>MNVDPHFDKFMESGIRHVYMLFENKSVESSEQFYSFMRTTYKNDPCSSDFECIERGAEMAQSYARIMNIKLETE[4x];>[4x]MEYYKQSKYETYSEIIEKERTARFESVALEQLQIVHISSEADFSAVYSFRPKNLNYFVDIIAYEGKLPSTISEKSLGGYPVDKTMDEYTV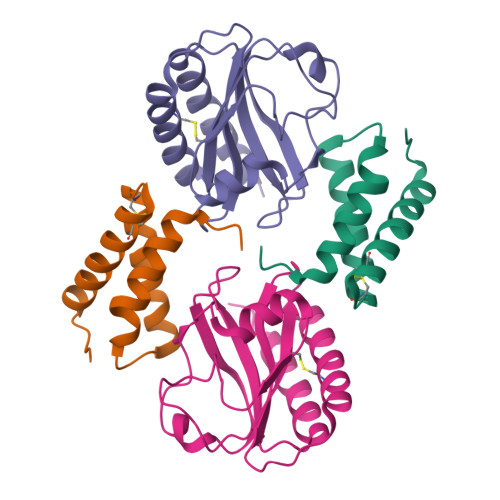HLNGRHYYSNSKFAFLPTKKPTPEINYMYSCPYFNLDNIYAGTITMYWYRNDHISNDRLESICAQAARILGRAK> MTCWL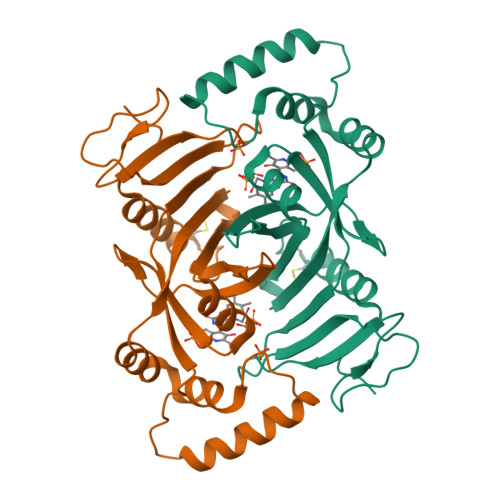RGVTATFGRPAEWPGYLSHLCGRSAAMDLGPMRKSYRGDREAFEETHLTSLDPVKQFAAWFEEAVQCPDIGEANAMCLATCTRDGKPSARMLLLKGFGKDGFRFFTNFESRKGKELDSNPFASLVFYWEPLNRQVRVEGPVKKLPEEEAECYFHSRPKSSQIGAVVSHQSSVIPDREYLRKKNEELEQLYQDQEVPKPKSWGGYVLYPQVMEFWQGQTNRLHDRIVFRRGLPTGDSPLGPMTHRGEEDWLYERLAP>[8x]MIDLNIMKVANYINGEFKEPSTGAFQVKTSPVDGSKIAEVPRSGREDAREAIDSAFEALKAWANIPAIRRAEYLYKMLE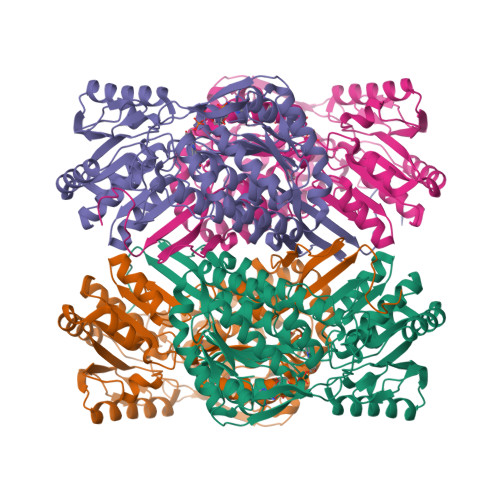VFRQMKEDFMKILTVEGGGTYRKVWGEVVFTERLIQNAAELARHYQGRVLQSDSESTISVVFKRSKGVVGVITPWNYPLSISMKKIAHTLAVGNTVVYKPASDTPVTGWLIAQMVAKAGLPKGVFNLVIGPGPVVGEEIVTHKRVAHVTFTGESSTGREIAAKAAGTLKTVTLELGGSDPLIILDDVDVDYAARLAVFASLFHQGQICTSAKRIIVHKAVADKFIERYVHYVKMLRIDDPRKDEKVDLGPLINERQVALMKEFVDDAVSRGGRLLIGGRSWGNFFEPAIFVDVDRNFRIMREEVFGPVRPIVVVENDDQAVEVANDTDYGLSGAVLTNNVNRAFRIAEAVESGMFHINDVTFLEESHVPFGGIKASGVGREGGEWSFHETTYDRWVTVTLRTRRFPIPSALK>[2x]AMADIVLSQIAICIWVESTAILQDCQRALSADRYQLQVCESGEMLLEYAQTHRDQIDCLILVAANPSFRAVVQQLCFEGVVVPAIVVGDRDSEDPDEPAKEQLYHSAELHLGIHQLEQLPYQVDAALAEFLRLAPVETMADHIMLMGANHDPELS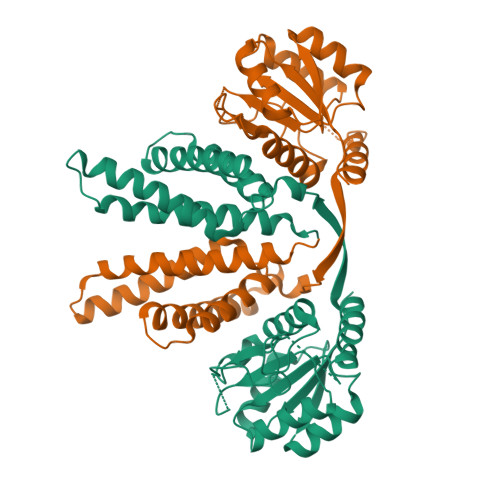SQQRDLAQRLQERLGYLGVYYKRDPDRFLRNLPAYESQKLHQAMQTSYREIVLSYFSPNSNLNQSIDNFVNMAFFADVPVTKVVEIHMELMDEFAKKLRVEGRSEDILLDYRLTLIDVIAHLCEMYRRSIPRET>[2x]ADTIVAVELDTYPNTDIGDPSYPHIGIDIKSVRSKKTAKWNMQNGKVGTAHI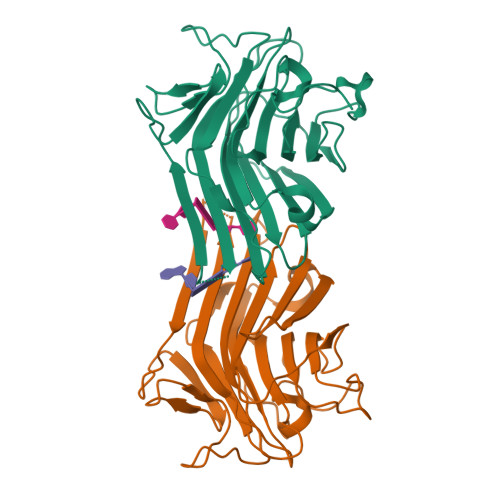IYNSVGKRLSAVVSYPNGDSATVSYDVDLDNVLPEWVRVGLSASTGLYKETNTILSWSFTSKLKSNSTHETNALHFVFNQFSKDQKDLILQGDATTGTDGNLELTRVSSNGSPQGSSVGRALFYAPVHIWESSAVVASFDATFTFLIKSSDSHPADGIAFFISNIDSSIPSGSTGRLLGLFPDAN>SNALFSVPVSDQEKAKDFYVETVGFDLLADQPGVHGRWLQVAPKGADTSLVLVDWFPTMPPGSLRGLLLRTDDVDADCARLQERGVAVDGPKNTPWG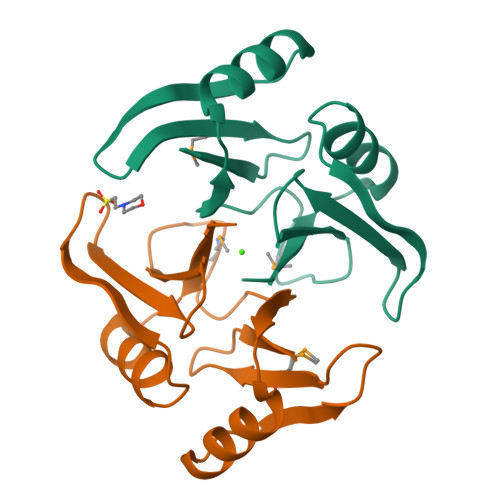RQAMFSDPDGNVIGLNQ[2x]> MHTAEFLETEPTEISSVLAGGYNHPLLRQWQSERQLTKNMLIFPLFISDNPDDFTEIDSLPNINRIGVNRLKDYLKPLVAKGLRSVILFGVPLIPGTKDPVGTAADDPAGPVIQGIKFIREYFPELYIICDVCLCEYTSHGHCGVLYDDGTINRERSVSRLAAVAVNYAKAGAHCVAPSDMIDGRIRDIKRGLINANLAHKTFVLSYAAKFSGNLYGPFRDAACSAPSNGDRKCYQLPPAGRGLARRALERDMSEGADGIIVK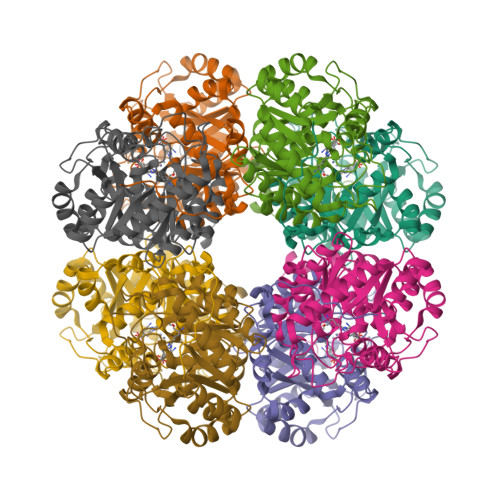PSTFYLDIMRDASEICKDLPICAYHVSGEYAMLHAAAEKGVVDLKTIAFESHQGFLRAGARLIITYLAPEFLDWLDEE>SRPVFKQVLKV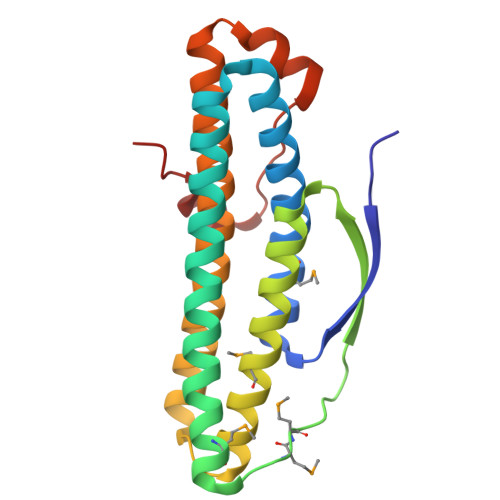NSLQAQRVMERSFERVSNSLFSIDVILRIIGEQDEIDQVETVILEHISKVSEDLDKATAQLNKLMEDNGIDMMPGYTNPNEYTIEINSPQVAQFAHLIRKLDTLMGIVDTLWLNTVLTSKQRTDATYQWQQRLIKLAGRIIGIEKRARISAHSKGKEGEVAEAAPESATGDKEIADEAEKTKA[2x]>SVYTYFSAVAGQDGEVDAEELQRCLTQSGINGTYSPFSLETCRIMIAMLDRDHTGKMGFNAFKELWAALNAWKENFMTVDQDGSGTVEHHELRQAIGLMGYRLSPQTLTTIVKRYSKNGRIFFDDYVACCVKLRALTDFFRKRDHLQQGSANFIYDDFLQGT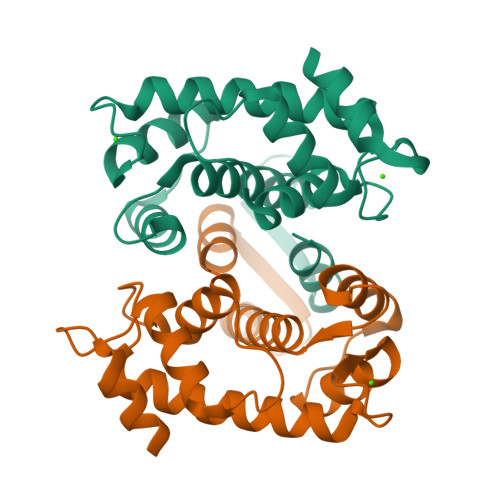MAI[2x]> MSGDENPASKPTPVQDVQGDGRWMSLHHRFVADSKDKEPEVVFIGDSLVQLMHQCEIWRELFSPLHALNFGIGGDSTQHVLWRLENGELEHIRPKIVVVWVGSNNHGHTAEQVTGGIKAIVQLVNERQPQARVVVLGLLPRGQHPNPLREKNRRVNELVRAALAGHPRAHFLDADPGFVHSD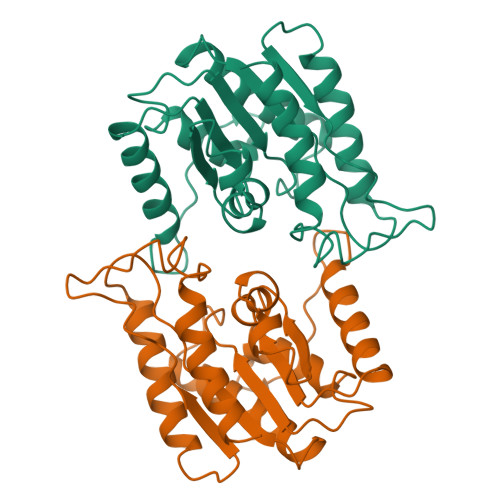GTISHHDMYDYLHLSRLGYTPVCRALHSLLLRLLTQDQGQGGAPLPEPSPP>[2x]ANPLYQKHIISINDLSRDDLNLVLATAAKLKANPQPELLKHKVIASCFFEASTRTRLSFETSMHRLGASVVGFSDSANTSLGKKGETLAD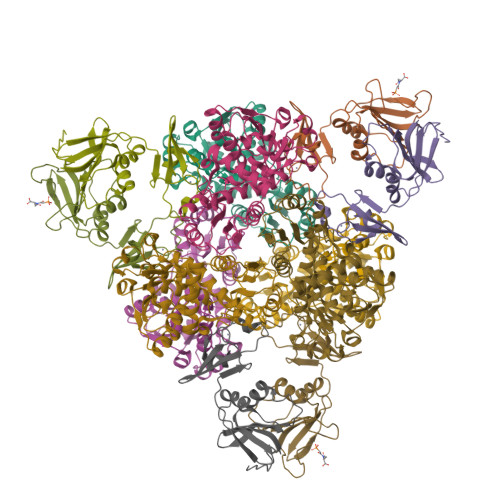TISVISTYVDAIVMAHPQEGAARLATEFSGNVPVLNAGDGSNQHPTQTLLDLFTIQETQGRLDNLHVAMVGDLKYGRTVHSLTQALAKFDGNRFYFIAPDALAMPQYILDMLDEKGIAWSLHSSIEEVMAEVDILYMTRVQKERLDPSEYANVKAQFVLRASDLHNAKANMKVLHPLPRVDEIATDVDKTPHAWYFQQAGNGIFARQALLALVLNRDLVL;>MTHDNKLQVEAIKRGTVIDHIPAQIGFKLLSLFKLTETDQRITIGLNLPSGEMGRKDLIKIENTFLSEDQVDQLALYAPQATVNRIDNYEVVGKSRPSLPERIDNVLVCPNSNCISHAEPVSSSFAVRKRANDIALKCKYCEKEFSHNVVLAN[2x]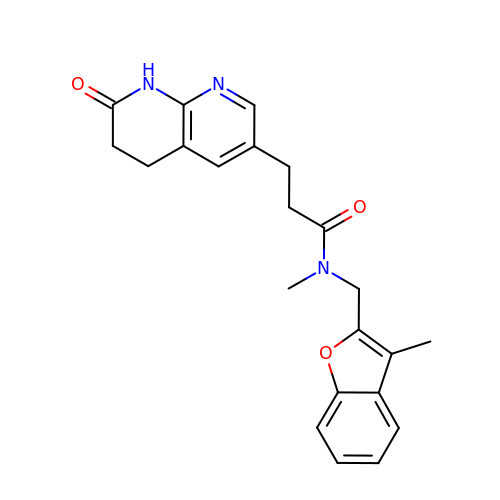N-methyl-N-[(3-methyl-1-benzofuran-2-yl)methyl]-3-(7-oxo-5,6,7,8-tetrahydro-1,8-naphthyridin-3-yl)propanamide | C22 H23 N3 O3 | WDNCPCMRTFYNIQ-UHFFFAOYSA-N> 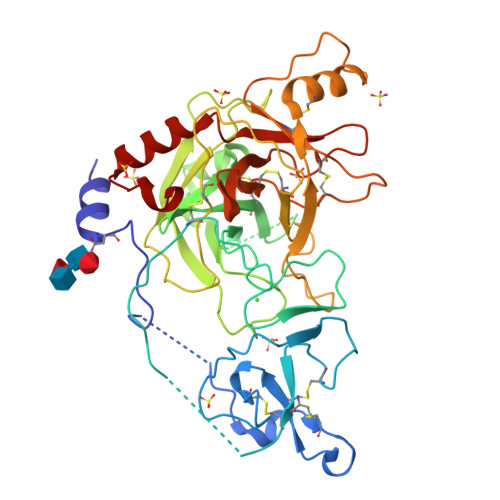GHMAVVNIFGNASEYIPPGYEIVTKAPLGALTALPRCGTGADQGKKVCIVYHRCDGVTNTVTPEEVINTTGEGIFDIRENANECESYLDVCCGLPEGGVLPTPSPTPPVVPVLKPSFCGIRNERGLDFKITGQTNEAEYGEFPWMVAVLKANVIPGSGEEQLVCGGSLIAPSVVLTGAHCVNSYQSNLDAIKIRAGEWDTLTEKERLPYQERKIRQVIIHSNFNPKTVVNDVALLLLDRPLVQADNIGTICLPQQSQIFDSTECFASGWGKKEFGSRHRYSNILKKIQLPTVDRDKCQADLRNTRLGLKFVLDQTFVCAGGEQGKDTCTGDGGSPLFCPDPRNPSRYMQMGIVAWGIGCGDENVPGVYANVAHFRNWIDQEMQAKGLSTTPYVE> MKVQYCDSLVIGGGLAGLRAAVATQQKGLSTIVLSLIPVKRSHSAAAQGGMQASLGNSKMSDGDNEDLHFMDTVKGSDWGCDQKVARMFVNTAPKAIRELAAWGVPWTRIHKGDRMAIINAQKTTITEEDFRHGLIHSRDFGGTKKWRTCYTADATGHTMLFAVANECLKLGVSIQDRKEAIALIHQDGKCYGAVVRDLVTGDIIAYVAKGTLIATGGYGRIYKNTTNAVVCEGTGTAIALETGIAQLGNMEAVQFHPTPLFPSGILLTEGCRGDGGILRDVDGHRFMPDYEPEKKELASRDVVSRRMIEHIRKGKGVQSPYGQHLWLDISILGRKHIETNLRDVQEICEYFAGIDPAEKWAPVLPMQHYSMGGIRTDYRGEAKLKGLFSAGEAACWDMHGFNRLGGNSVSEAVVAGMIVGEYFAEHCANTQVDLETKTLEKFVKGQEAYMKSLVESKGTEDVFKIKNRMKDVMDDNVGIFRDGPHLEKAVKELEELYKKSKNVGIKNKRLHANPELEEAYRVPMMLKVALCVAKGALDRTESRGAHNREDYPKRDDINWLNRTLASWPNPEQTLPTLEYEALDVNEMEIAPGYRGYGAKGNYIENPLSVKRQEEIDKIQSELEAAGKDRHAIQE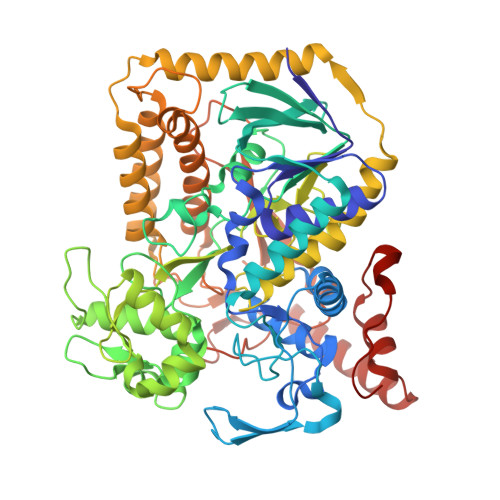ALMPYELPAKYKARNERLGDK αHBs are oligomers of 5 or more α-helical peptides that assemble into coiled-coil structures with central solvent-accessible channels. We targeted two properties of αHBs: oligomeric state, which directly affects the internal diameter of the channel; and the identities of channel-facing residues, which fine tune this dimension and introduce different chemistries. The αHBs are loaded with an environment sensitive dye (in this case, 1,6-diphenyl-1,3,5-hexatriene, DPH) that binds within the channels and fluoresces. Accordingly, challenging the array with analytes leads to differential displacement of the dye across the array to give a fluorescent fingerprint.

Despite the requirements for aliphatic residues at a and d, up to 40% of these can be changed to other side chains without compromising barrel integrity. We introduced mutations at one or two of these sites to generate four groups of αHB: Group I had entirely hydrophobic interiors, but with different sizes and shapes of channel; Groups II and III had polar uncharged or polar charged residues, respectively, at specific points along the channel; and Group IV had aromatic residues installed in their channels. The eleven Group II peptides comprised: single mutants to Cys, His, Asn, Ser or Thr at d sites; and double mutations to His, Asn, Ser or Thr at consecutive a and d sites. Finally, one third of the designs were crystallized and yielded 12 X-ray crystal structures, all of which were open αHBs with fully accessible channels. Focusing on the small molecules, the αSA signal from the more-polar AAs and CHOs is dominated by the polar and charged Group II and III αHBs.

>[2x]XGEIAQALKEIAKALKEIAWALKENAQALKGX>[4x]ASIFGVFDIKTDAVELRKKALELSRLMRHRGPDWSGIYASDNAILAHERLSIVDVNAGAQPLYNQQKTHVLAVNGEIYNHQALRAEYGDRYQFQTGSDCEVILALYQEKGPEFLDDLQGMFAFALYDSEKDAYLIGRDHLGIIPLYMGYDEH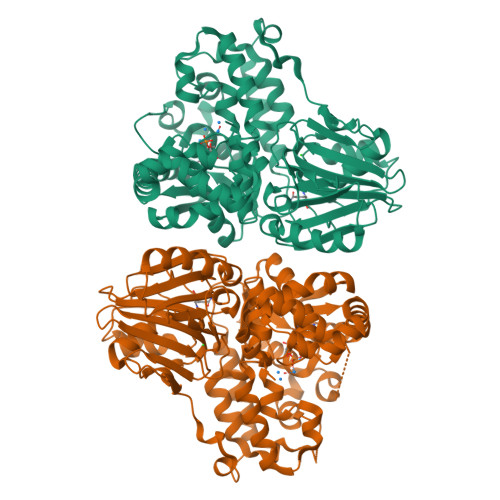GQLYVASEMKALVPVCRTIKEFPAGSYLWSQDGEIRSYYHRDWFDYDAVKDNVTDKNELRQALEDSVKSHLMSDVPYGVLLSGGLDSSIISAITKKYAARRVEDQERSEAWWPQLHSFAVGLPGSPDLKAAQEVANHLGTVHHEIHFTVQEGLDAIRDVIYHIETYDVTTIRASTPMYLMSRKIKAMGIKMVLSGEGSDEVFGGYLYFHKAPNAKELHEETVRKLLALHMYDCARANKAMSAWGVEARVPFLDKKFLDVAMRINPQDKMCGNGKMEKHILRECFEAYLPASVAWRQKEQFSDGVGYSWIDTLKEVAAQQVSDQQLETARFRFPYNTPTSKEAYLYREIFEELFPLPSAAECVPGGPSVACSSAKAIEWDEAFKKMDDPSGRAVGVHQSAYK>MTIAVTGSIATDHLMRFPGRFSEQLLPEHLHKVSLSFLVDDLVMHRGGVAGNMAFAIGVLGGEVALVGAAGADFADYRDWLKARGVNCDHVLISETAHTARFTCTTDVDMAQIASFYPGAMSEARNIKLADVVSAIGKPELVIIGANDP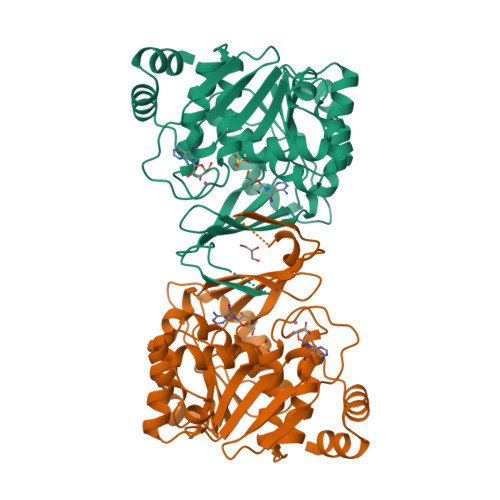EAMFLHTEECRKLGLAFAADPSQQLARLSGEEIRRLVNGAAYLFTNDYEWDLLLSKTGWSEADVMAQIDLRVTTLGPKGVDLVEPDGTTIHVGVVPETSQTDPTGVGDAFRAGFLTGRSAGLGLERSAQLGSLVAVLVLESTGTQEWQWDYEAAASRLAGAYGEHAAAEIVAVLA[2x]>[4x]MKHMPRKMYSCAFETTTKVEDCRVWAYGYMNIEDHSEYKIGNSLDEFMAWVLKVQADLYFHNLKFAGAFIINWLERNGFKWSADGLPNTYNTIISRMGQWYMIDICLGYKGKRKIHTVIYDSLKKLPFPVKKIAKDFKLTVLKGDIDYHKERPVGYKITPEEYAYIKNDIQIIAEALLIQFKQGLDRMTAGSDSLKGFKDIITTKKFKKVFPTLSLGLDKEVRYAYRGGFTWLNDRFKEKEIGEGMVFDVNSLYPAQMYSRLLPYGEPIVFEGKYVWDEDYPLHIQHIRCEFELKEGYIPTIQIKRSRFYKGNEYLKSSGGEIADLWLSNVDLELMKEHYDLYNVEYISGLKFKATTGLFKDFIDKWTYIKTTSEGAIKQLAKLMLNSLYGKFASNPDVTGKVPYLKENGALGFRLGEEETKDPVYTPMGVFITAWARYTTITAAQACYDRIIYCDTDSIHLTGTEIPDVIKDIVDPKKLGYWAHESTFKRAKYL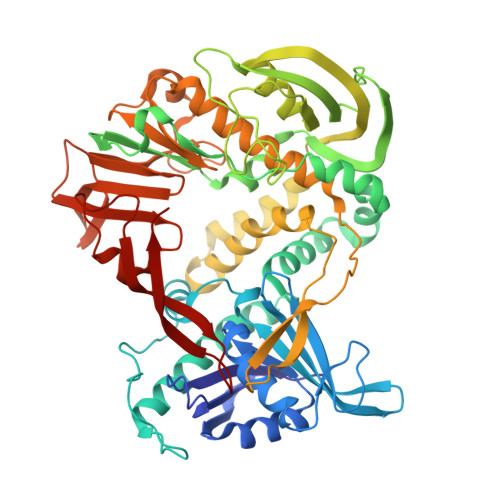RQKTYIQDIYMKEVDGKLVEGSPDDYTDIKFSVKCAGMTDKIKKEVTFENFKVGFSRKMKPKPVQVPGGVVLVDDTFTIK> AGLNKDQKRRAEQLTSIFENGTTEIQYGYVERLDDGRGYTCGRAGFTTATGDALEVVEVYTKAVPNNKLKKYLPELRRLAKEESDDTSNLKGFASAWKSLANDKEFRAAQDKVNDHLYY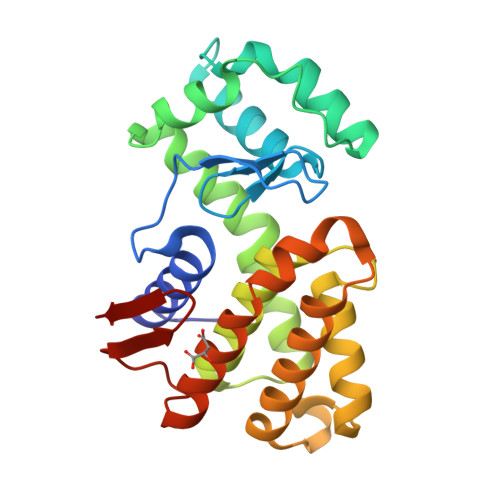QPAMKRSDNAGLKTALARAVMYDTVIQHGDGDDPDSFYALIKRTNKKAGGSPKDGIDEKKWLNKFLDVRYDDLMNPANHDTRDEWRESVARVDVLRSIAKENNYNLNGPIHVRSNEYGNFVIK> F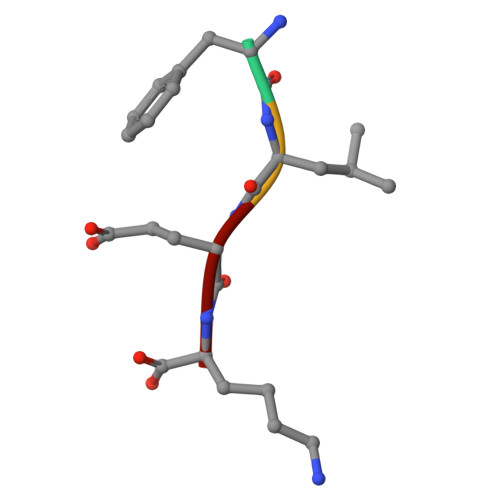LEK Autophagosome formation is a fundamental process in macroautophagy/autophagy, a conserved self-eating mechanism in all eukaryotes, which requires the conjugating ATG (autophagy related) protein complex, ATG12–ATG5-ATG16L1 and lipidated MAP1LC3/LC3 (microtubule associated protein 1 light chain 3). Here, we demonstrated that RAB33B plays a key role in recruiting the ATG16L1 complex to phagophores during starvation-induced autophagy. Crystal structures of RAB33B bound to the coiled-coil domain (CCD) of ATG16L1 revealed the recognition mechanism between RAB33B and ATG16L1. ATG16L1 is a novel RAB-binding protein (RBP) that can induce RAB proteins to adopt active conformation without nucleotide exchange.

We prepared the ATG16L1(141–265) complexes with GDP-bound RAB33B(30–218) or GTP-bound RAB33BQ92L(30–218). Their crystal structures were determined at 2.4 Å. In both structures, GTP- and GDP-bound RAB33B-ATG16L1 complexes adopt the same conformation. The complex showed a dyad symmetry with a 2:2 configuration. Two molecules of ATG16L1(141–265) formed a homodimer, within which the dimeric helices of ATG16L1 formed a parallel coiled-coil structure (residues 161–194). The C-terminal segments of two helices (residues 195–225) are detached from each other, where one RAB33B molecule binds independently to each helix. Each RAB33B bound one molecule of GTP or GDP and one Mg2+ with well-defined electron density. RAB33B interacted with ATG16L1 mainly through its switch I, switch II and inter switch regions, whereas both the CCD and the C-terminal detached helices of ATG16L1 homodimer were involved in the binding with RAB33B. The core hydrophobic interaction formed by invariant, hydrophobic dyad residues of I66 and F95 in the switch regions of RAB33BA molecule (molecule A of the dimeric complex) with W194 and V191 in the CCD of ATG16L1A molecule, respectively. L205 of ATG16L1 made hydrophobic contacts with F70 and W87, two of invariant, hydrophobic triad residues of RABs (F70, W87 and Y103), which have been proposed to be important for RAB-effector interactions.

>GPMRSRIFKIIVIGDSNVGKTCLTYRFCAGRFPDRTEATIGVDFRERAVEIDGERIKIQLWDTAGLERFRKSMVQHYYRNVHAVVFVYDMTNMASFHSLPSWIEECKQHLLANDIPRILVGNKCDLRSAIQVPTDLAQKFADTHSMPLFETSAKNPNDNDHVEAIFMTLAHKLKSHKPLMLSQPPDNGIILK[2x];>[2x]MLETNCLDLRTKLQDLEVANQTLKDEYDALQITFTALEEKLRKTTEENQELVTRWMAEKAQEANRLNAENEKDSRRRQARLQKELAEAAKEPLPVEQDDDIEVIVDETSDHTEETSPVRAVSRAAT>MARSVRVLVDMDGVLADFEAGLLRGFRRRFPEEPHVPLEQRRGFLARE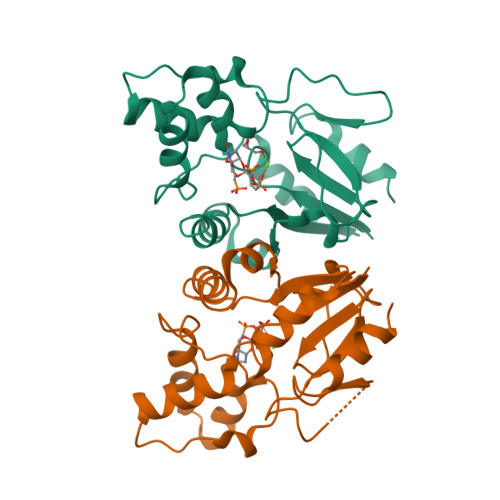QYRALRPDLADKVASVYEAPGFFLDLEPIPGALDAVREMNDLPDTQVFICTSPLLKYHHCVGEKYRWVEQHLGPQFVERIILTRDKTVVLGDLLIDDKDTVRGQEETPSWEHILFTCCHNRHLVLPPTRRRLLSWSDNWREILDSKR[2x]>[2x]SPHVFISYSWSSEDHKEWVLDLANKLMKESGVEVIL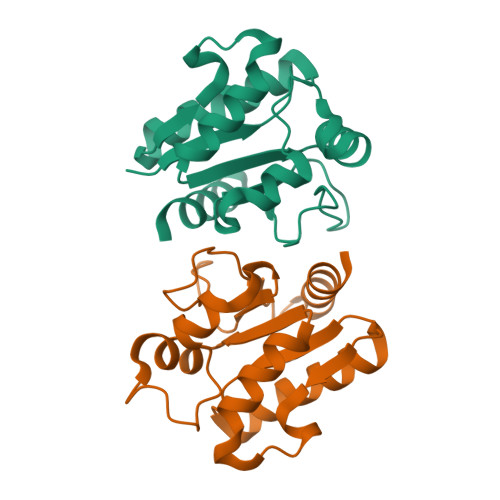DRWHGVVGHDRFEFMENSIKIADKVLVICDKDYCEKANTRRGGVGTETMIITPNIYNNTKQEKFIPISLGEENGEYFLPDFFKSRFALGWNYEDIDKSYKELERLIWE> MGSMTL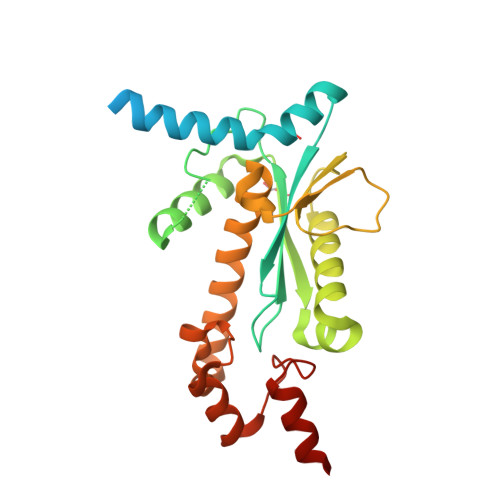TIKEVTQLINAVNTIEELENHECFLDERKGVQNAIARRRKALEKEQALKEKYVEMTYFENEILKEHPNAIICGIDEVGRGPLAGPVVACATILNSNHNYLGLDDSKKVPVTKRLELNEALKNEVTAFAYGIATAEEIDEFNIYKATQIAMQRAIDGLSVQPTHLLIDAMTLDNALPQVSLIKGDARSVSIAAASIMAKVFRDDYMTQLSKDYPEYGFEKNAGYGTKQHLLAIDDIGIMKEHRKSFEPIKSLLLEHHHHHH(1R,3S,Z)-5-(2-((3aS,7aS,E)-1-(6-hydroxy-6-methylhept-1-en-1-ylidene)-7a-methyloctahydro-4H-inden-4-ylidene)ethylidene)-4-methylenecyclohexane-1,3-diol 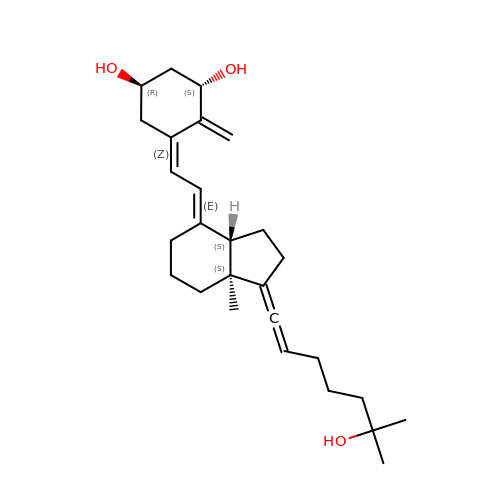| C27 H40 O3 | ZUEJBGWNHJHNIO-PIOXGFLRSA-N> GSHMLPRETDEEPEEPGRRGSFVEMVDNLRGKSG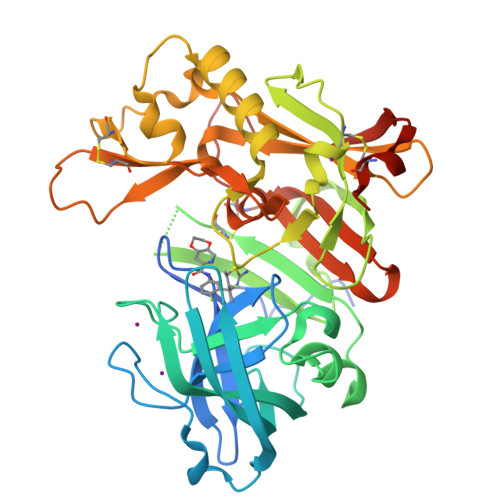QGYYVEMTVGSPPQTLNILVDTGSSNFAVGAAPHPFLHRYYQRQLSSTYRDLRKGVYVPYTQGKWEGELGTDLVSIPHGPNVTVRANIAAITESDKFFINGSNWEGILGLAYAEIARPDDSLEPFFDSLVKQTHVPNLFSLQLCGAGFPLNQSEVLASVGGSMIIGGIDHSLYTGSLWYTPIRREWYYEVIIVRVEINGQDLKMDCKEYNYDKSIVDSGTTNLRLPKKVFEAAVKSIKAASSTEKFPDGFWLGEQLVCWQAGTTPWNIFPVISLYLMGEVTNQSFRITILPQQYLRPVEDVATSQDDCYKFAISQSSTGTVMGAVIMEGFYVVFDRARKRIGFAVSACHVHDEFRTAAVEGPFVTLDMEDCGYNIPQTDEST>[3x]MALYREGKAAMAADGTVTGTGTKWQSSLSLIRPGATIMFLSSPIQMAVVNKVVSDTEIKAITTNGAVVASTDYAILLSDSLTVDGLAQDVAETLRYYQSQETVIADAVEFFKEFDFESLQNLANQIKADSEASESSAAAAAASESKAKTSEDNAKSSENAAKNSEVAAETTRDQIQQIIDNAGDQSTLVVLAQPDGFDSIGRVSSFAALRNLKPKKSGQHVLLTSYYDGWAAENKMPTGGGEFISSIGTATDDGGYIAAGPGYYWTRVVNNNSFTAEDFGCKTTATPPPNFNVLPAELFDNTARMQAAFNLAISKSFKLNLS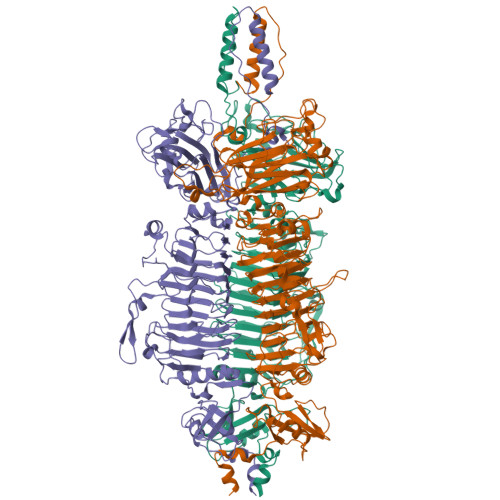AGTYYFESSDTLRITGPIHIEGRPGTVFYHNPSNKANPKTDAFMNISGCSMGRISSINCFSNSYLGKGINFDRSVGDNRKLVLEHVYVDTFRWGFYVGEPECINQIEFHSCRAQSNYFQGIFIESFKEGQEYGHSAPVHFFNTICNGNGPTSFALGATYKTTKNEYIKVMDSVNDVGCQAYFQGLSNVQYIGGQLSGHGSPRNTSLATITQCNSFIIYGTDLEDINGFTTDGTAITADNIDTIESNYLKDISGAAIVVSSCLGFKIDSPHIFKIKTLSTIKLMNNTYNYEIGGFTPDEALKYNVWDANGLATNRISGVIHPRLVNSRLGINSVAFDNMSNKLDVSSLIHNETSQIIGLTPSTGSNVPHTRIMWSNGAMYSSTDLNNGFRLNYLSNHNEPLTPMHLYNEFSVSEFGGSVTESNALDEIKYIFIQTTYANSGDGRFIIQALDASGSVLSSNWYSPQSFNSTFPISGFVRFDVPTGAKKIRYGFVNSANYTGSLRSHFMSGFAYNKRFFLKIYAVYNDLGRYGQFEPPYSVAIDRFRVGDNTTQMPSIPASSATDVAGVNEVINSLLASLKANGFMSS>MGLASLADFPIGVAVAASGGNADIFTSSARQNIVRAEFNQITAENIMKMSYMYSGSNFSFTNSDRLVSWAAQNGQTVHGHTLVWHPSYQLPNWASDSNANFRQDFARHIDTVAAHFAGQVKSWDVVNEALFDSADDPDGRGSANGYRQSVFYRQFGGPEYIDEAFRRARAADPTAELYYNDFNTEENGAKTTALVNLVQRLLNNGVPIDGVGF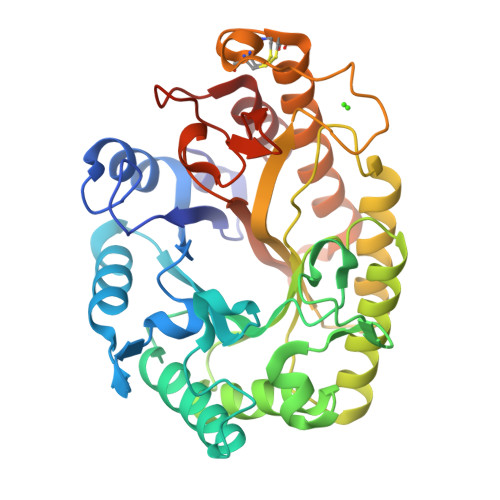QMHVMNDYPSIANIRQAMQKIVALSPTLKIKITELDVRLNNPYDGNSSNEYTNRNDCAVSCAGLDRQKARYKEIVQAYLEVVPPGRRGGITVWGIADPDSWLYTHQNLPDWPLLFNDNLQPKPAYQGVVEALSGR[2x]>[3x]MEPHVLGAGLYWLLLPCTLLAASLLRFNALSLVYLLFLLLLPWLPGPSRHSIPGHTGRLLRALLCLSLLFLVAHLAFQICLHTVPHLDQFLGQNGSLWVKVSQHIGVTRLDLKDIFNTTRLVAPDLGVLLASSLCLGLCGRLTRKAGQSRRTQELQDDDDDDDDDDEDIDAAPAVGLKGAPALATKRRLWLASRFRVTAHWLLMTSGRTLVIVLLALAGIAHPSAFSSIYLVVFLAICTWWSCHFPLSPLGFNTLCVMVSCFGAGHLICLYCYQTPFIQDMLPPGNIWARLFGLKNFVDLPNYSSPNALVLNTKHAWPIYVSPGILLLLYYTATSLLKLHKSCPSELRKETPREDEEHELELDHLEPEPQARDATQGEMPMTTEPDLDNCTVHVLTSQSPVRQRPVRPRLAELKEMSPLHGLGHLIMDQSYVCALIAMMVWSIMYHSWLTFVLLLWACLIWTVRSRHQLAMLCSPCILLYGLTLCCLRYVWAMELPELPTTLGPVSLHQLGLEHTRYPCLDLGAMLLYLLTFWLLLRQFVKEKLLKKQKVPAALLEVTVADTEPTQTQTLLRSLGELVTGIYVKYWIYVCAGMFIVVSFAGRLVVYKIVYMFLFLLCLTLFQVYYTLWRKLLRVFWWLVVAYTMLVLIAVYTFQFQDFPTYWRNLTGFTDEQLGDLGLEQFSVSELFSSILIPGFFLLACILQLHYFHRPFMQLTDLEHVPPPGTRHPRWAHRQDAVSEAPLLEHQEEEEVFREDGQSMDGPHQATQVPEGTASKWGLVADRLLDLAASFSAVLTRIQVFVRRLLELHVFKLVALYTVWVALKEVSVMNLLLVVLWAFALPYPRFRPMASCLSTVWTCIIIVCKMLYQLKIVNPHEYSSNCTEPFPNNTNLQPLEINQSLLYRGPVDPANWFGVRKGYPNLGYIQNHLQILLLLVFEAVVYRRQEHYRRQHQQAPLPAQAVCADGTRQRLDQDLLSCLKYFINFFFYKFGLEICFLMAVNVIGQRMNFMVILHGCWLVAILTRRRREAIARLWPNYCLFLTLFLLYQYLLCLGMPPALCIDYPWRWSKAIPMNSALIKWLYLPDFFRAPNSTNLISDFLLLLCASQQWQVFSAERTEEWQRMAGINTDHLEPLRGEPNPIPNFIHCRSYLDMLKVAVFRYLFWLVLVVVFVAGATRISIFGLGYLLACFYLLLFGTTLLQKDTRAQLVLWDCLILYNVTVIISKNMLSLLSCVFVEQMQSNFCWVIQLFSLVCTVKGYYDPKEMMTRDRDCLLPVEEAGIIWDSICFFFLLLQRRIFLSHYFLHVSADLKATALQASRGFALYNAANLKSINFHRQIEEKSLAQLKRQMKRIRAKQEKYRQSQASRGQLQSKDPQDPSQEPGPDSPGGSSPPRRQWWRPWLDHATVIHSGDYFLFESDSEEEEEALPEDPRPAAQSAFQMAYQAWVTNAQTVLRQRRERARQERAEQLASGGDLNPDVEPVDVPEDEMAGRSHMMQRVLSTMQFLWVLGQATVDGLTRWLRAFTKHHRTMSDVLCAERYLLTQELLRVGEVRRGVLDQLYVGEDEATLSGPVETRDGPSTASSGLGAEEPLSSMTDDTSSPLSTGYNTRSGSEEIVTDAGDLQAGTSLHGSQELLANARTRMRTASELLLDRRLHIPELEEAERFEAQQGRTLRLLRAGYQCVAAHSELLCYFIIILNHMVTASAASLVLPVLVFLWAMLTIPRPSKRFWMTAIVFTEVMVVTKYLFQFGFFPWNSYVVLRRYENKPYFPPRILGLEKTDSYIKYDLVQLMALFFHRSQLLCYGLWDHEEDRYPKDHCRSSVKDREAKEEPEAKLESQSETGTGHPKEPVLAGTPRDHIQGKGSIRSKDVIQDPPEDLKPRHTRHISIRFRRRKETPGPKGTAVMETEHEEGEGKETTERKRPRHTQEKSKFRERMKAAGRRLQSFCVSLAQSFYQPLQRFFHDILHTKYRAATDVYALMFLADIVDIIIIIFGFWAFGKHSAATDIASSLSDDQVPQAFLFMLLVQFGTMVIDRALYLRKTVLGKLAFQVVLVVAIHIWMFFILPAVTERMFSQNAVAQLWYFVKCIYFALSAYQIRCGYPTRILGNFLTKKYNHLNLFLFQGFRLVPFLVELRAVMDWVWTDTTLSLSNWMCVEDIYANIFIIKCSRETEKKYPQPKGQKKKKIVKYGMGGLIILFLIAIIWFPLLFMSLIRSVVGVVNQPIDVTVTLKLGGYEPLFTMSAQQPSIVPFTPQAYEELSQQFDPYPLAMQFISQYSPEDIVTAQIEGSSGALWRISPPSRAQMKQELYNGTADITLRFTWNFQRDLAKGGTVEYTNEKHTLELAPNSTARRQLAQLLEGRPDQSVVIPHLFPKYIRAPNGPEANPVKQLQPDEEEDYLGVRIQLRREQVGTGASGEQAGTKASDFLEWWVIELQDCKADCNLLPMVIFSDKVSPPSLGFLAGYGIVGLYVSIVLVVGKFVRGFFSEISHSIMFEELPCVDRILKLCQDIFLVRETRELELEEELYAKLIFLYRSPETMIKWTRERE

Piezo ion channels, Piezo1 and Piezo2, are mechanosensitive channels (MS channels) that underlie force-detection in eukaryotic cells. The number of cellular processes found mediated by Piezo channels is large and growing at a rapid rate. Their essential biophysical characteristics include responsiveness in gating to mechanical force (i.e. mechanosensitivity) and selectivity of the pore for cations. Biophysical studies suggest that Piezo channels sense force directly through the lipid membrane, although other mechanisms also have been proposed. Viewed down its 3-fold axis, the trimeric Piezo channel is a triskelion with extended arms; from the side, it is curved as shown.

Using cryo-electron microscopy (cryo-EM) we determined a structure of mPiezo1 to an overall resolution of 3.7 Å. The refined structural model contains 1518 residues (out of 2547), with the N-terminal 576 residues and internal flexible loops missing. The structure’s extended arms consist of 24 helices arranged as six repeated 4-TM structural units. The six 4-TM repeats assemble with each other also as a left-handed helix, causing the extended arms of the triskelion to spiral away from the trimer’s center, out of plane with respect to the central pore axis. At the center TM37-38 form a 3-fold symmetric channel lined by TM38, capped on the extracellular side by a CED, and extended on the intracellular side by a pore extension (PE) helix. The cuff consists of ‘elbow’ helices (residues 2116 to 2142), a ‘base’ helix (residues 2149 to 2175) and ‘hairpin' helices (residues 2501 to 2534) from all three subunits. The transmembrane pore, lined by TM38 and the PE helix, is closed. At the level of the membrane inner leaflet, the pore radius at positions E2537, P2536 and M2493 is 0.1 Å, 0.4 Å and 0.3 Å, respectively. However, the detergent micelle containing a trimer is curved into a dome shape. A negatively charged patch of amino acids (E2257, E2258 and D2264) on the CED lies in close contact with a positively charged patch (R1761, R1762 and R1269) located in the extracellular loops of 4-TM units 2 and 3.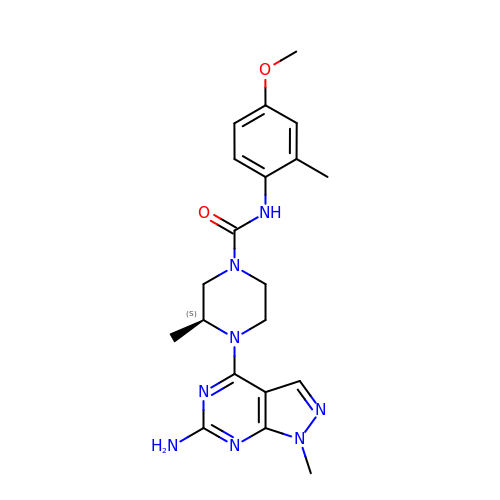(3~{S})-4-(6-azanyl-1-methyl-pyrazolo[3,4-d]pyrimidin-4-yl)-~{N}-(4-methoxy-2-methyl-phenyl)-3-methyl-piperazine-1-carboxamide | C20 H26 N8 O2 | WRONAJQPZWDYAR-ZDUSSCGKSA-N> GKITFYEDRGFQGHCYESSSDCPNLQPYFSRCNSIRVDSGCWMLYERPNYQGHQYFLRRGDYPDYQQWMGFNDSIRSCRLIPQHTGTFRMRIYERDDFRGQMSEITDDCPSLQDRFHLTEVHSLNVLEGSWVLYEMPSYRGRQYLLRPGEYRRYLDWGAMNAKVGSLRRV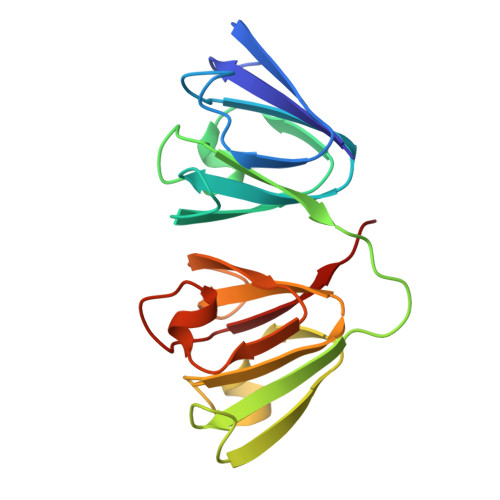MDFY>[2x]QEVRRGDFVRNWQLVAAVPLFQKLGPAVLVEIVRALRARTVPAGAVICRIGEPGDRMFFVVEGSVSVATPNPVELGPGAFFGEMALISGE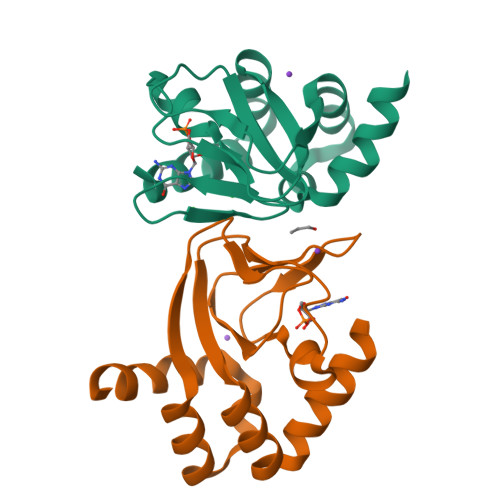PRSATVSAATTVSLLSLHSADFQMLCSSSPEIAEIFRKTALERRGAAASA>[2x]MSTSSSSQSLKIGIVGFGNFGQFLAKTMIKQGHTLTATSRSDYSELCLQMGIHFFRDVSAFLTADIDVIVLCTSILSLSEVVGSMPLTSLKRPTL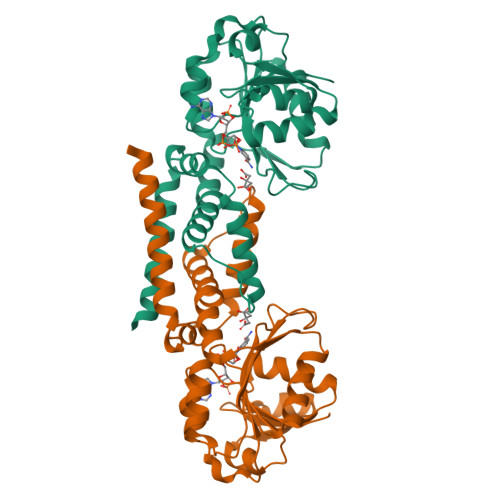FVDVLSVKEHPRELLLRELPEDSDILCTHPMFGPQTAKNGWTDHTFMYDKVRIRDEVICSNFIQIFATEGCKMVQMSCEEHDRAAAKSQFITHTIGRTLGEMDIQSTPIDTKGFETLVKLKETMMRNSFDLYSGLFVYNRFARQELENLEHALHKVKETLMIQRTNGEQGHKRTES> XGFGVVP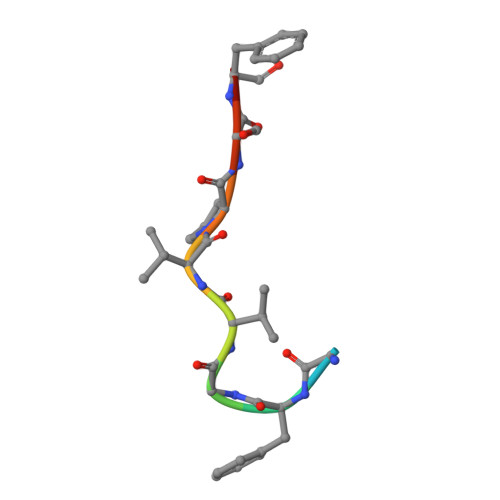SFY> GPGHMVVKFSYMWTINNFSFCREEMGEVIKSSTFSSGANDKLKWCLRVNPKGLDEESKDYLSLYLLLVSCPKSEVRAKFKFSIL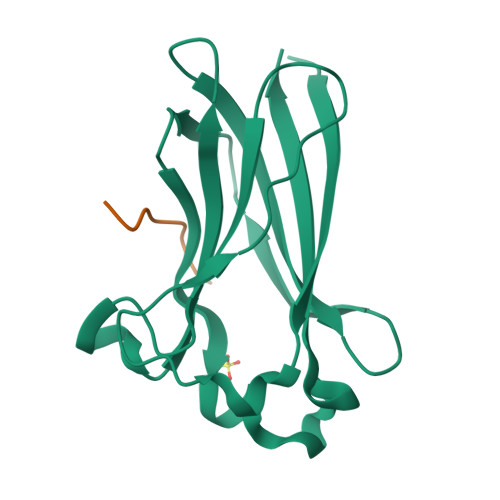NAKGEETKAMESQRAYRFVQGKDWGFKKFIRRGFLLDEANGLLPDDKLTLFCEVSVVQD;> PATPTASSSSSTTPT EQUILIN | C18 H20 O2 | 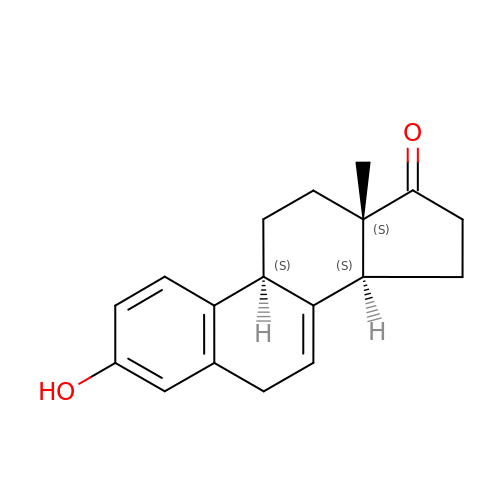WKRLQDKEXYKHJB-HFTRVMKXSA-N> GAMESLPVIAAPSMWTRPQIKDFKEKIQQDADSVITVGRGEVVTVRVPTHEEGSYLFWEFATDNYDIGFGVYFEWTDSPNTAVSVHVSESSDDDEEEEENIGCEEKAKKNANKPLLDEIVPVYRRDCHEEVYAGSHQYPGRGVYLLKFDNSYSLWRSKSVYYRVYYTR;> GSGSGTPAPDAINDALRSADSQEARDACQKKGWIVIHPSNELVVEKHISR

ACBD3 is a Golgi resident protein involved in the maintenance of the Golgi structure and regulation of intracellular trafficking between the endoplasmic reticulum and the Golgi. However, in enterovirus-infected cells, the ACBD3 GOLD domain interacts preferentially with viral non-structural 3A proteins, which causes re-localization of ACBD3 to the sites of virus replication. In this study, we present a structural, biochemical, and biological characterization of the complexes composed of human ACBD3 and the 3A proteins of four representative enteroviruses. The crystal structures revealed the details of the ACBD3-3A interaction, the 3A-3A interaction causing the assembly of the ACBD3-3A heterotetramers, the interaction between the ACBD3-3A complex and the lipid bilayer, and the roles of these interactions in facilitation of enterovirus replication.

To analyze the dimerization of the GOLD: 3A complexes in more detail, we generated a mutant EVD68 3A protein (hereafter referred to as LVVY mutant) with the following four mutations at the putative dimerization interface: L25A, V29A, V34A, and Y37A. Taking advantage of the vicinity of the C terminus of the ACBD3 GOLD domain and the N terminus of the ordered part of the EVD68 3A protein, we connected the last residue of ACBD3 (R528ACBD3) through a short peptide linker (GSGSG) to the first ordered residue of the EVD68 3A protein (T163A/EVD68). Both GOLD-3A wild-type and LVVY mutant fusion proteins formed crystals, which diffracted to a resolution suitable for further structure determination. The crystal structures of the GOLD: 3A complex consisting of two individual proteins, the GOLD-3A fusion protein, and its LVVY mutant were almost identical with low root-median-square deviations, confirming that neither the fusion-protein approach nor the LVVY mutation affected the correct folding of these proteins. Three lines of evidence document the dimeric state of the wild-type GOLD-3A fusion protein and the monomeric state of its LVVY mutant in vitro. Secondly, the small-angle X-ray scattering (SAXS) profiles of these proteins correspond to the calculated scattering curves of a dimer of the wild-type GOLD-3A fusion protein and of a monomer of its LVVY mutant. Thirdly, crystal contacts corresponding to the 3A dimerization interface are not preserved in the crystal structure of the GOLD-3A LVVY mutant, indicating that this mutant cannot dimerize through this interface even at very high protein concentrations (of approximately 20 mM) present within the protein crystal. Nevertheless, we observed a significant difference in FRET efficiency between the wild-type GOLD-3A fusion protein and its LVVY mutant. Finally, we analyzed the impact of the LVVY mutation on enterovirus replication. Using a reporter subgenomic replicon assay for EVD68 established earlier, we found replication of this mutant significantly attenuated in both U-87 MG and HaCaT cells.4-[bis(4-chlorobenzyl)amino]-N-hydroxybutanamide | C18 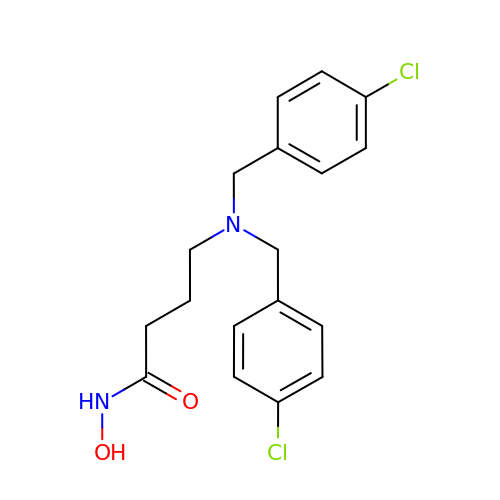H20 Cl2 N2 O2 | DFRQCUSEVBJDPJ-UHFFFAOYSA-N>[2x]QSACTLQSETHPPLTWQKCSSGGTCTQQTGSVVIDANW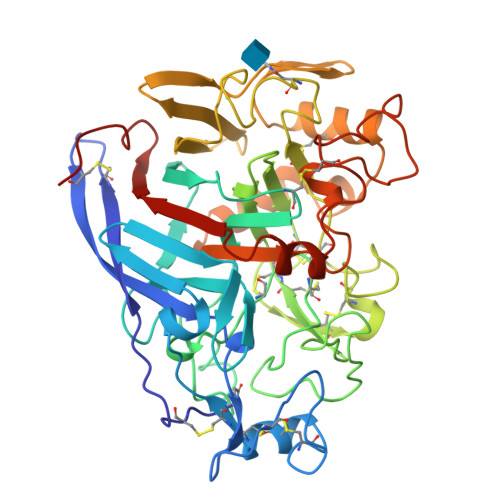RWTHATNSSTNCYDGNTWSSTLCPDNETCAKNCCLDGAAYASTYGVTTSGNSLSIDFVTQSAQKNVGARLYLMASDTTYQEFTLLGNEFSFDVDVSQLPCGLNGALYFVSMDADGGVSKYPTNTAGAKYGTGYCDSQCPRDLKFINGQANVEGWEPSSNNANTGIGGHGSCCSQMDIWEANSISEALTPHPCTTVGQEICEGDGCGGTYSDNRYGGTCDPDGCDWNPYRLGNTSFYGPGSSFTLDTTKKLTVVTQFETSGAINRYYVQNGVTFQQPNAELGSYSGNELNDDYCTAEEAEFGGSSFSDKGGLTQFKKATSGGMVLVMSLWDDYYANMLWLDSTYPTNETSSTPGAVRGSCSTSSGVPAQVESQSPNAKVTFSNIKFGPIGSTGNPSG>MFSAGHKIKGTVVLMPKNELEVNPDGSAVDNLNAFLGRSVSLQLISATKADAHGKGKVGKDTFLEGINTSLPTLGAGESAFNIHFEWDGSMGIPGAFYIKNYMQVEFFLKSLTLEAISNQGTIRFVCNSWVYNTKLYKSVRIFFANHTYVPSETPAPLVEYREEELKSLRGNGTGERKEYDRIYDYDVYNDLGNPDKSEKLARPVLGGSSTFPYPRRGRTGRGPTVTDPNTEKQGEVFYVPRDENLGHLKSKDALEIGTKSLSQIVQPAFESAFDLKSTPIEFHSFQDVHDLYEGGIKLPRDVISTIIPLPVIKELYRTDGQHILKFPQPHVVQVSQSAWMTDEEFAREMIAGVNPCVIRGLEEFPPKSNLDPAIYGDQSSKITADSLDLDGYTMDEALGSRRLFMLDYHDIFMPYVRQINQLNSAKTYATRTILFLREDGTLKPVAIELSLPHSAGDLSAAVSQVVLPAKEGVESTIWLLAKAYVIVNDSCYHQLMSHWLNTHAAMEPFVIATHRHLSVLHPIYKLLTPHYRNNMNINALARQSLINANGIIETTFLPSKYSVEMSSAVYKNWVFTDQALPADLIKRGVAIKDPSTPHGVRLLIEDYPYAADGLEIWAAIKTWVQEYVPLYYARDDDVKNDSELQHWWKEAVEKGHGDL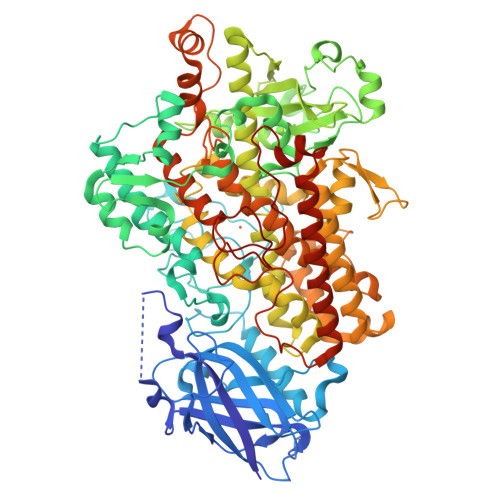KDKPWWPKLQTLEDLVEVCLIIIWIASALHAAVNFGQYPYGGLIMNRPTASRRLLPEKGTPEYEEMINNHEKAYLRTITSKLPTLISLSVIEIASTHASDEVYLGQRDNPHWTSDSKALQAFQKFGNKLKEIEEKLVRRNNDPSLQGNRLGPVQLPYTLLYPSSEEGLTFRGIPNSISI[2x]>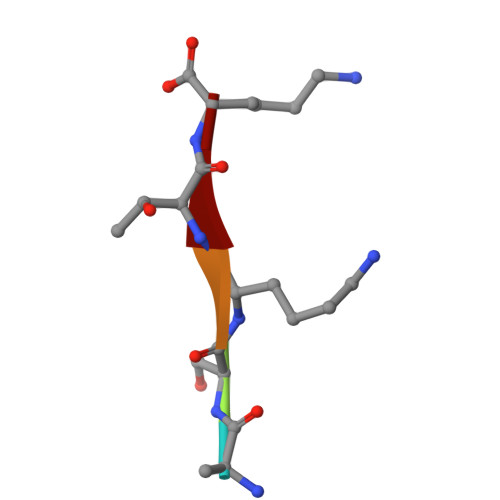 ASKTK>[2x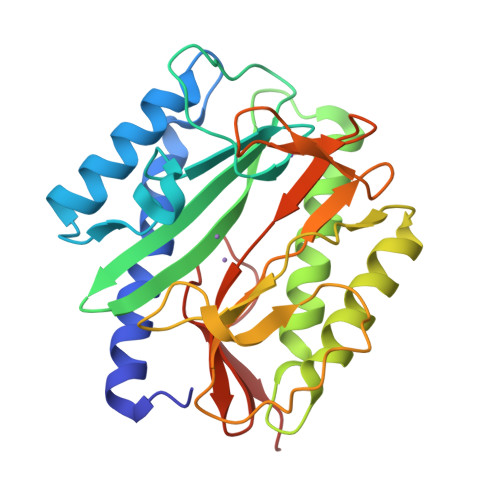]ASSIKTPEDIEKMRVAGRLAAEVLEMIEPYVKPGVSTGELDRICNDYIVNEQHAVSACLGYHGYPKSVCISINEVVCHGIPDDAKLLKDGDIVNIDVTVIKDGFHGDTSKMFIVGKPTIMGERLCRITQESLYLALRMVKPGINLREIGAAIQKFVEAEGFSVVREYCGHGIGRGFHEEPQVLHYDSRETNVVLKPGMTFTIEPMVNAGKKEIRTMKDGWTVKTKDRSLSAQYEHTIVVTDNGCEILTLRKDDTIPAIISHDE>[2x]MSKDFDLIIRNAYLSEKDSVYDIGIVGDRIIKIEAKIEGTVKDEIDAKGNLVSPGFVDAHTHMDKSFTSTG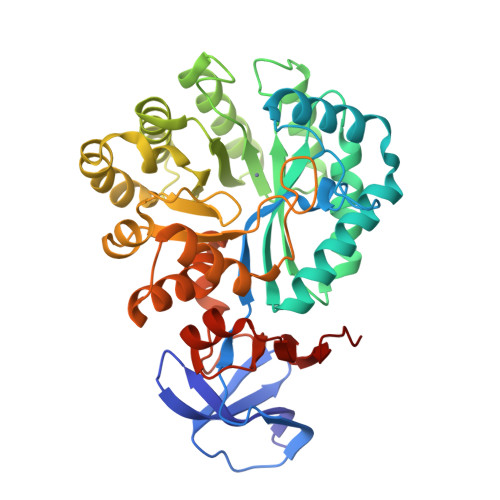ERLPKFWSRPYTRDAAIEDGLKYYKNATHEEIKRHVIEHAHMQVLHGTLYTRTHVDVDSVAKTKAVEAVLEAKEELKDLIDIQVVAFAQSGFFVDLESESLIRKSLDMGCDLVGGVDPATRENNVEGSLDLCFKLAKEYDVDIDYHIHDIGTVGVYSINRLAQKTIENGYKGRVTTSHAWCFADAPSEWLDEAIPLYKDSGMKFVTCFSSTPPTMPVIKLLEAGINLGCASDNIRDFWVPFGNGDMVQGALIETQRLELKTNRDLGLIWKMITSEGARVLGIEKNYGIEVGKKADLVVLNSLSPQWAIIDQAKRLCVIKNGRIIVKDEVIVA>AQSVPYGISQIKAPALHSQGYTGSNVKVAVIDSGIDSSHPDLNVRGGASFVPSETNPYQDGSSHGTHVAGTIAALNNSIGVLGVAPSASLYAVKVLDSTGSGQYSWIINGIEWAISNNMDVINMSLGGPSGSTALKTVVDKAVSSGIVVAAAAGNEGSSGSSSTVGYP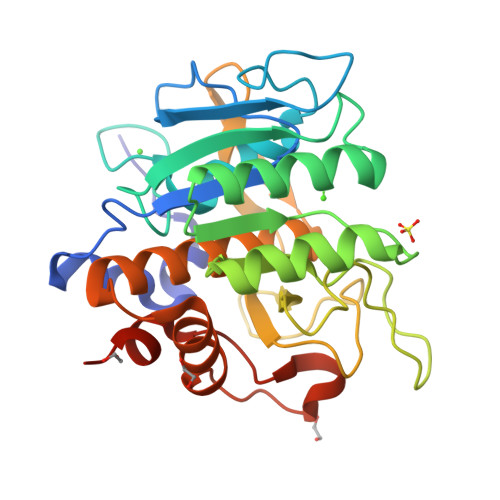AKYPSTIAVGAVNSSNQRASFSSAGSELDVMAPGVSIQSTLPGGTYGAYNGTCMATPHVAGAAALILSKHPTWTNAQVRDRLESTATYLGNSFYYGKGLINVQAAAQSLEHHHHHH[2x]> MPHSLFSTDTDLTAENLLRLPAEFGCPVWVYDAQIIRRQIAALKQFDVVRFAQKACSNIHILRLMREQGVKVDSVSLGEIERALAAGYNPQTHPDDIVFTADVIDQATLERVSELQIPVNAGSVDMLDQLGQVSPGHRVWLRVNPGFGHGHSQKTNTGGENSKHGIWYTDLPAALDVIQRHHLQLVGIHMHIGSGVDYAHLEQVCGAMVRQVIEFG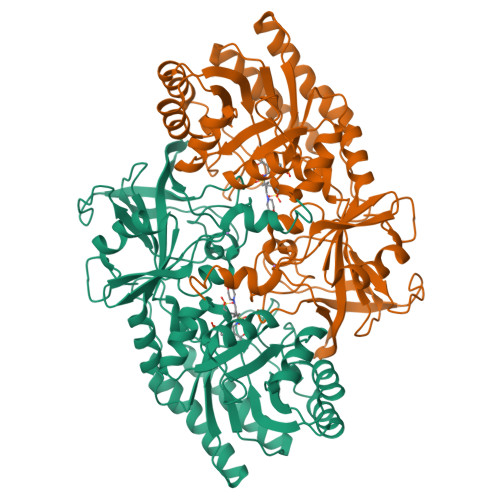QDLQAISAGGGLSVPYQQGEEAVDTEHYYGLWNAAREQIARHLGHPVKLEIEPGRFLVAQSGVLITQVRSVKQMGSRHFVLVDAGFNDLMRPAMYGSYHHISALAADGRSLEHAPTVETVVAGPLCESGDVFTQQEGGNVETRALPEVKAGDYLVLHDTGAYGASMSSNYNSRPLLPEVLFDNGQARLIRRRQTIEELLALELLHHHHH>GARDVQEGVSSFEESGGAQLPPRVHALEVLEGAGPGRLHGRLGIKPDGQPGYTRAPSPPTDLSMPQALARGGGFNLYLSDHLELDRTAPDARHASCRQLHYDLSTLPKASVIIVFYNEPFSTLMRSVHSVLNGTPPQILEELILVDDGSTLPYIREDGNQQLVEYLKLLPAKVRLIRNEVRKGIVGARMKGIRASRAPIFAILDSHIEVSPQWLEPLLLRIKEDSRRVVMPQIDGIDAETFKHIAGGIGCKLGFLWKLMEHSYEGHQTARLPPEERQPSPTDFQTSPAMAGGLFAANKAFFFDVGAYDEDFQFWGTENLELSFRLWQCGGVLECAPCSRVYHIFRKGGSGYSSPGDSITINKMRTMLWMDEYADLAWRVIGKPRVNYRPESLEKRREWRKRKGCKSFRWFMENVFPEGDVVTLDDVPYLGPLRNDKIGMCLDNMGWASPGHAVGLEYCHGGDTQTFMFFRKVGHVMPVNDDEACLQPSGRLDWCRGTAQFWWDFTSSGQLMFRETKQCLSAFGRKLRMVECDDTDPYQIWSWTAYNPPDTFTFPSVSRSIRSG[2x];> GTTPSPVPTTSTTSAP

O-glycosylation of the protein CST1 by the mucin-type O-glycosyltransferase T. gondii (Txg) GalNAc-T3 influences cyst wall rigidity and stability. The strict glycopeptide-preferring enzyme TxgGalNAc-T3 then adds GalNAc to acceptor Thr one position N-terminal to existing Thr-O-GalNAcs and is predicted to sequentially O-glycosylate Thr rich repeats within the mucin domain of CST1. The structures reveal a unique GalNAc binding pocket that dictates the substrate preference of TxgGalNAc-T3, which is coupled to a 2nd metal binding site that is strictly conserved among apicomplexan homologs.

To investigate the basis of the substrate specificity and function of TxgGalNAc-T3, we solved the x-ray co-crystal structures of TxgGalNAc-T3 in complex with Mn2+, a non-hydrolysable form of UDP-GalNAc (UDP-2-(acetylamino)−4-F-D-galactosamine disodium salt, UDP-GalNAc-F) and each of the following glycopeptides: CST1.4, Muc5AC-3,13, Muc5AC-3, Muc5AC-13, and SRS13.2 from 2.2-2.9 Å resolution. We modeled UDP into the active site but did not include GalNAc-F due to weak electron density, either due to the high mobility of the GalNAc moiety or hydrolysis of UDP-GalNAc-F during crystallization. For the mono-glycopeptides, we observe density for Thr-O-GalNAc in the TxgGalNAc-T3:Muc5AC-3 co-crystal structure, but disconnected and weak density for the peptide residues. Overall, the lack of density for the peptide backbone or Thr-O-GalNAc at the C-terminal ends of the glycopeptides suggests a lack of strong interactions with the catalytic or lectin domain of TxgGalNAc-T3. Thr-O-GalNAc at the +1 position on the glycopeptides is bound to a pocket in TxgGalNAc-T3 consisting of His333 (catalytic domain) and Glu554 (lectin domain) that interact with GalNAc via sidechain H-bonds, and Ser334 (catalytic domain), which interacts with GalNAc through a mainchain H-bond. We observed density that appears to be a 2nd metal (Mn2+N) near the GalNAc binding pocket, a striking and unexpected feature not previously seen in metazoan GalNAc-Ts.> HHHHHHHHSQAGDTLNDVIQDPTRRNKLINDNNLLKGIIMGRDGPVPSSRELIVRPDTLRAIINNRATIETTTMEAEFTETLMESNYNSASVKVSAPFITANSEYSESSSFKNTETEKSMYTSSRYLFPQGRIDFTTPDSGFDDVIKLSPQFTSGVQAALAKATGTEKREALQNLFQEYGHVFRTKVHIGGVLSAHTMETFSRSENETEVKQDVKAGLEGAVKGWGGGATAGHGNTQGTITTSQNRKLNVKYIVNVVDYTKIQNTEEWVASTNQSEHWRVIEVTEVTAVADLLPQPIRGQVKDLLKPLLGKWVDVEKVPGLESLPVSVYRPKGAIPAGWFWLGDTADASKALLVKPTLPARSGRNPALTSLH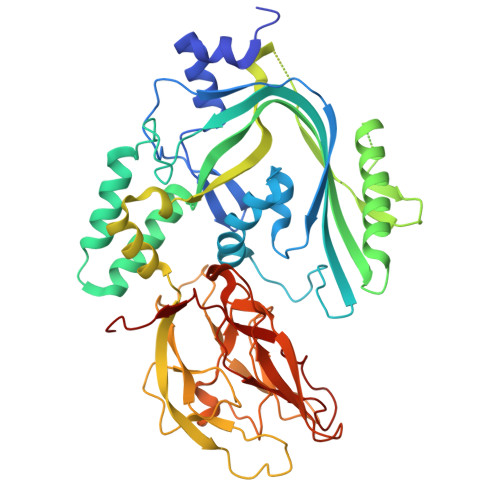QGSGMTEQPFVDLPQYQYLSTYFGSFAHDTPPGSTLRGLRPDHVLPGRYEMHGDTISTAVYVTRPVDVPFPEDECFDLKSLVRVKLPGSGNPPKPRSALKKSMVLFDSGEK>[5x]SNAMIIRPEQHWFLRLFDWHGSVLSKIIFRLLLNVLMSIIAIISYQWYEQLGIHLTVAPFSLLGIAIAIFLGFRNSASYSRFVEARNLWGTVL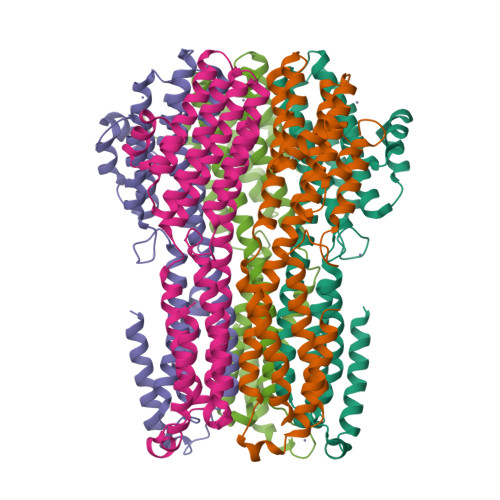IAERTLVRQLRNILPAEHDAHRRIVSYLVAFSWSLKHQLRKTDPTADLRRLLPEERVTEILASSMPTNRILLLAGNEIGQLREAGKTSDITYGLMDNKLDELAHVLGGCERLATTPVPFAYTLILQRTVYLFCTLLPFALVGDLHYMTPFVSVFISYTFLSWDSLAEELEDPFGTAANDLPLNAMCNTIERNLLDMTGQHPLPE>[2x]MPVKFHTKTLESVIDPVAQQVGQLVLFHEQAESGLLKEDLTPLVQGVGIAVTNLVQVAASMVETSNDEDFKAELPPSMQEVQQAAVFLSDAARLLKADQGSPEGKRKLLDGARGVINGMSDLLMCADRSEVRKMVKVCRSVQEYLDVAKVIDVEADLATFLQNLTPGMTSMMKVVEQRHPELTNLAHAQMLKSELGTVREQIPILISSIRVCCLVIVKDGSSGMKDAAFGRDYVIQKLFIAIEEIIRVLQLTTTFEEEEVGGAGAASAASLAHMFHQAQDALASGDISRSTLDAVRKCISEGRRVA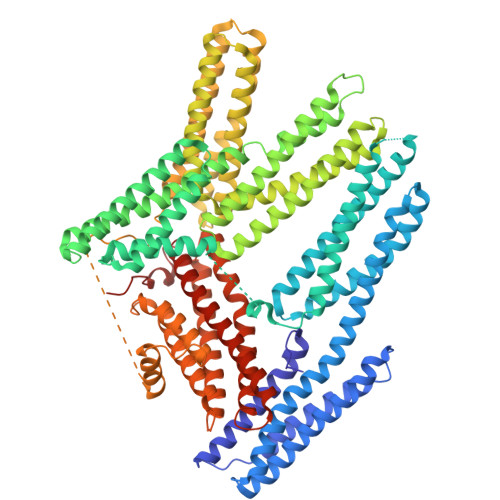ALAATDETRAKLLAAADELDQILKELEELQAKGLGDSRQARALAHAAAVKLQELEQEIRKALAERVATDFVNVGGPIKALEDAALASPSDPNRQANFAQKAKEFEAHTARLADTAELVASSGGCSDAVAAELRKEAAKLRDISTAVVPAARVVLENPGNQAAKDYLRTVKEKWLEAAESMGRSVDGVIDSLEFMKVSEARIQADVKEAKRIALAEEDSMKLIAKASSVARQANRVIQVAKVEADNSENPEFVAKLSSASESLAKSISPMVIEAKAVVTSPQNKDIQRKFCSSADKVVEGVAAVRSVIEDNWVPPRPPLPELEEEEEPPELPPPPEDPASLLPAEMQEAEEMLRAPLPPKDQNPIHHAAASVFREADQWDEKGNDLISLVKQMARKMAMMSKYTRGESGEVRSKADLIRMAKEIALNAQELLKLARQIANACMDKRAKTNLLQLLDRIPTISTQLKILATVKATSMGGGDARADADATDMLVGNAENLMRTVKDVIRASEAACIRLRPDSPIASILWRKKGGQGRRISVSY>[2x]VEHPEFLKAGKEPGLQIWRVEKFDLVPVPTNLYGDFFTGDAYVILKTVQLRNGNLQYDLHYWLGNECSQDESGAAAIFTVQLDDYLNGRAVQHREVQGFESATFLGYFKSGLKYKKGGVASGFKHVVPNEVVVQRLFQVKRRRVVRATEVPVSWESFNNGDCFILDLGNNIHQWCGSNSNRYERLKATQVSKGIRDNERSGRARVHVSEEGTEPEAMLQVLGPKPALPAGTEDTAKEDAANRKLAKLYKVSNGAGTMSVSLVADENPFAQGALKSEDCFILDHGKDGKIFVWKGKQANTEERKAALKTASDFITKMDYPKQTQVSVLPEGGETPLFKQFFKNWRDPDQTDGLGLSYLSSHIANVERVPFDAATLHTSTAMAAQHGMDDDGTGQKQIWRIEGSNKVPVDPATYGQFYGGDSYIILYNYRHGGRQGQIIYNWQGAQSTQDEVAASAILTAQLDEELGGTPVQSRVVQGKEPAHLMSLFGGKPMIIYKGGTSRE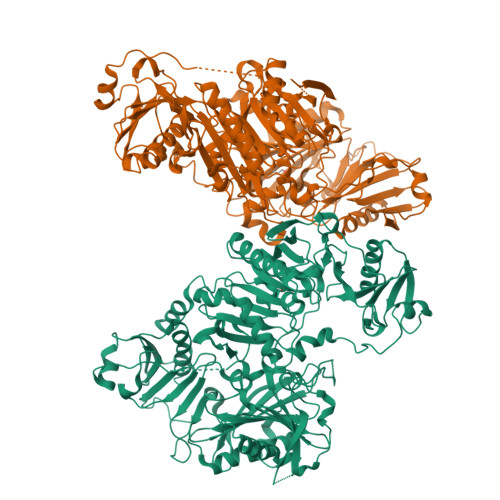GGQTAPASTRLFQVRANSAGATRAVEVLPKAGALNSNDAFVLKTPSAAYLWVGTGASEAEKTGAQELLRVLRAQPVQVAEGSEPDGFWEALGGKAAYRTSPRLKDKKMDAHPPRLFACSNKIGRFVIEEVPGELMQEDLATDDVMLLDTWDQVFVWVGKDSQEEEKTEALTSAKRYIETDPANRDRRTPITVVKQGFEPPSFVGWFLGWDDDYWSVDPLDRAMAELAA>[6x]DNQHKKIKGY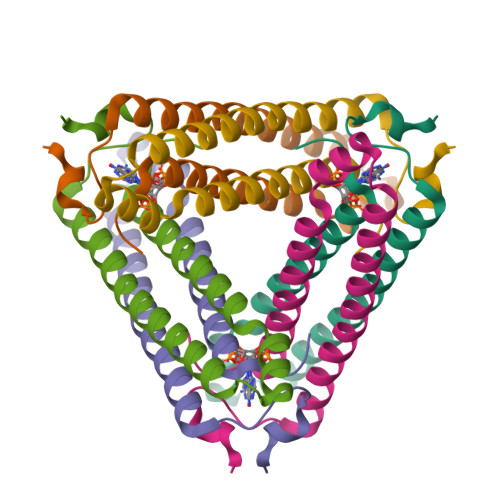RDLSQEEIDMMNRVKELGSQFEKLIQDVSDHLRGQYNASLHNRDEITRIANAEPGRWLAIGKTDIQTGMMAIIRAIAQPDSF>MSITLRTYIFLDALQPQLATFIGKTARGFLPVPGQASLWVEIAPGIAINRVTDAALKATKVQPAVQVVERAYGLLEVHHFDQGEVLAAGSTILDKLEVREEGRLKPQVMTHQIIRAVEAYQTQIINRNSQGMMILPGESLFILETQPAGYAVLAANEAEKAANVHLVNVTPYGAFGRLYLAGSEAEIDAAAEAAEAAIRSVSGVAQESFRDR[6x];>MADALGMIEVRGFVGMVEAADAMVKAAKV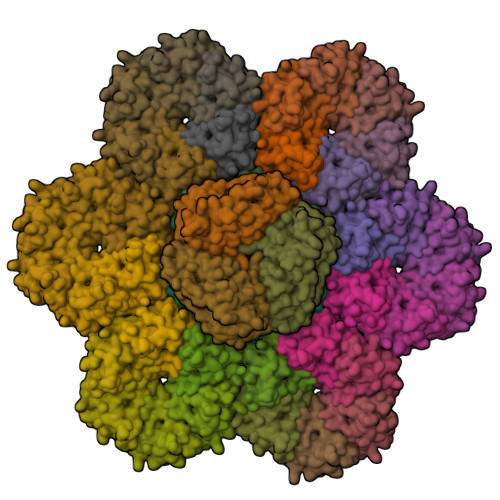ELIGYEKTGGGYVTAVVRGDVAAVKAATEAGQRAAERVGEVVAVHVIPRPHVNVDAALPLGRTPGMDKSA[36x]> MPSTYKTPGVYIEEISKFPPSIAQVETAIPAFIGYTQIAKVGVENFHTDADNLILRPVRITSLLEYEQFFGKAINETTIQVVIQDTTDSRGNLTERKASARITSPSPHNLYYSMQAYFANGGGPCYIVSVGPMSNTGTIQLEALQNGLAEVAKEDEVTLLVFPESQSLSDENYAALMSAALEQCANLQDRFTVMDLKLPATRPIPANAIVGASNAFRDLSLPQDNLKYGACYAPDIETIFNYFYQEDAVTIFRSVNGGAEEQDTLTMAGYNPANGGDGIQYALIESAIDQLPLILPPSPLVVGQYARTDNTRGVWKAPANVALSSVIKPVLKITNEQQNNLNVHPTGKSINAIRAFTGKGTLIWGARTLAGNDNEWRYVSVRRFFNMAEESIKKGSEPFVFEPNDANTWTKVKAMIENFLTLQWRAGALAGAKPEQAFYVKIGLNETMTALDILEGRMIVEIGMAVVRPAEFII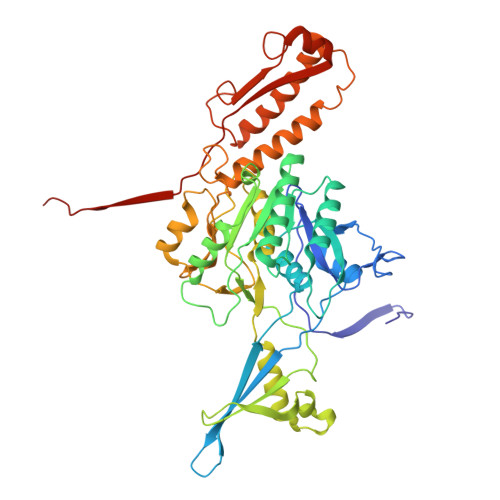LKFSHKMQES N-({(2S)-1-[(3R)-3-AMINO-4-(2-FLUOROPHENYL)BUTANOYL]PYRROLIDIN-2-YL}METHYL)BENZAMIDE | C22 H26 F N3 O2 | 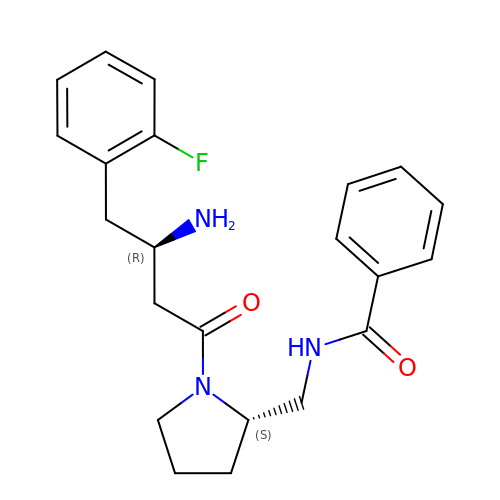ANQHSFFUNMTTRS-MOPGFXCFSA-N>[2x]MNAQAEEFKKYLETNGIKPKQFHKKELIFNQWDPQEYCIFLYDGITKLTSISENGTIMNLQYYKGAFVIMSGFIDTETSVGYYNLEVISEQATVYVIKINELKELLSKNLTHFFYVFQTLQKQVSYSLAKFNDFSINGKLGSICGQLLILTYVYGKETPDGIKITLDNLTMQELGYSSGIAHSSAVSRIISKLKQEKVIVYKNSCFYVQNLDYLKRYAPKLDEWFYLACPATWGKLN

The major regulator of virulence factors in L. monocytogenes is the transcription activator PrfA, a member of the Crp/Fnr family of regulators. PrfAWT is a homodimer in which each monomer consists of an N-terminal domain (residues 1 to 108) and a C-terminal DNA-binding domain (residues 138 to 237) linked by a long α-helix (αC, residues 109 to 137). Two α-helices in the C-terminal domain, αE (residues 170 to 178) and αF (residues 183 to 197), constitute the two helices of the typical HTH motif present in many prokaryotic transcription factors. Glutathione binding stabilizes the DNA-binding helix-turn-helix (HTH) motif in a conformation compatible with DNA-binding, thereby allowing expression of PrfA-regulated virulence factors.

In addition, we found three new PrfA mutants in the remaining three strains—Leu to His substitution at residue 140 (PrfAL140H), Ala to Gly substitution at residue 218 (PrfAA218G), and Ala to Val substitution at residue 94 (PrfAA94V). All the previously identified PrfA* mutants, i.e., PrfAG145S, PrfAG145C, and PrfAL140F, could grow in this medium with G-6-P, as could the PrfA mutants PrfAL140H and PrfAA218G, whereas the strain carrying the PrfAA94V mutation was unable to grow. The results were consistent with the fosfomycin sensitivity test—all the prfA mutant strains showed significantly increased hpt expression compared to the wild-type strain, with the A94V substitution having a minute increase in hpt expression. Based on these data, we hypothesize that the original A94V transposon mutant carried a secondary site mutation, allowing it to grow in medium having G-6-P as the sole carbon source. Hence, the new mutant structures display features characteristic of both the inactive and active forms of PrfA. It is noteworthy that we did not manage to get crystals of the PrfAWT under these crystallization conditions; however, crystals of PrfAA94V, which showed almost PrfAWT activity levels, were obtained. The PrfAA94V protein also had one folded HTH and one unfolded (WT) motif identical to that of the PrfA* mutants. Thus, the new structures of PrfA* variants and the wild-type-like PrfAA94V protein, presented here, represent an intermediately activated form of the protein. The most striking structural difference between the inactive, intermediate-active, and fully active structures is the position of their recognition helices. When superimposed on monomer B, the recognition helix in monomer A is shifted up to 6 Å.>[4x]MTPSHPARPSRSGILVFDVNETLL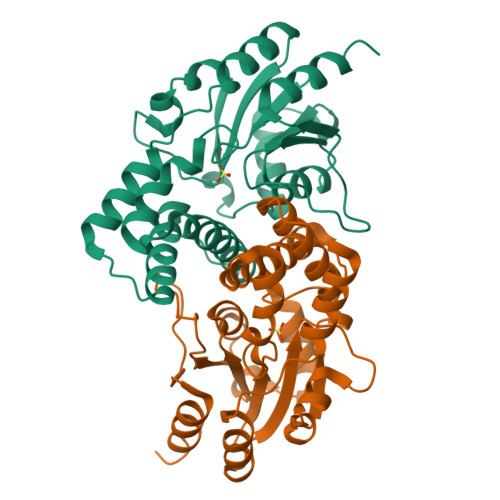DLTSLSPLFERVFGDAKVLREWFPELILYSQTLTLTGLYRPFGEIAAAVFEMVAANHQAKVTPDDIAELKTRLTSMPAYPDVAPALTRLQDAGFRLVTLTNSAPSPAPSPLEKAGIASFFEAHLTVHSSQRFKPHPSVYDSTAETLGAKPEELCMIACHIWDTIGAQARGWRGGFVARPHNTPLTLAEVPQPDFIGRDMGELADQLIASLTA> SSPPVVDTVHGKVLGKFVSLEGFAQPVAIFLGIPFAKPPLGPLRFTPPQPAEPWSFVKNATSYPPMCTQDPKAGQLLSELFTNRKENIPLKLSEDCLYLNIYTPADLTKKNRLPVMVWIHGGGLMVGAASTYDGLALAAHENVVVVTIQYRLGIWGFFSTGDEHSRGNWGHLDQVAALRWVQDNIASFGGNPGSVTIFGESAGGESVSVLVLSPLAKNLFHRAISESGVALTSVLVKKGDVKPLAEQIAITAGCKTTTSAVMVHCLRQKTEEELLETTLKMKFLSLDLQGDPRESQPLLGTVIDGMLLLKTPEELQAERNFHTVPYMVG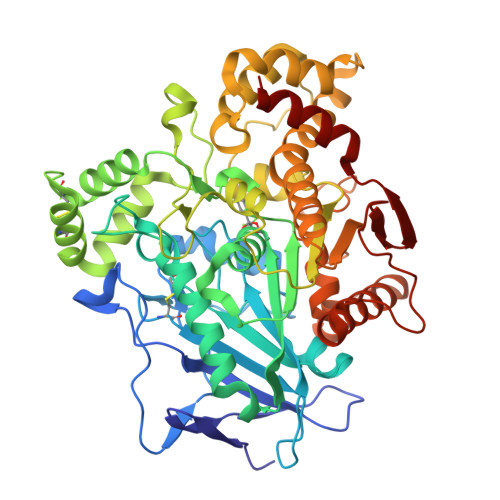INKQEFGWLIPMQLMSYPLSEGQLDQKTAMSLLWKSYPLVCIAKELIPEATEKYLGGTDDTVKKKDLFLDLIADVMFGVPSVIVARNHRDAGAPTYMYEFQYRPSFSSDMKPKTVIGDHGDELFSVFGAPFLKEGASEEEIRLSKMVMKFWANFARNGNPNGEGLPHWPEYNQKEGYLQIGANTQAAQKLKDKEVAFWTNLFAK>SHMQCIVNACKNSWDKSYLAGTPNKDNCSGFVQSVAAELGVPMPRGNANAMVDGLEQSWTKLASGAEAAQKAAQGFLVIAGLKGRTYGHVAVVISGPLYRQKYPMCWCGSIAGAVGQSQGLKSVGQVWNRTDRDRLNYYVYSLASC[2x];>[2x]ADCTFTQLEIVPQFGSPNMFGGEDEHVRVMFSNEDPNDDNPDAFPEPPVYLADRDSGNDCRIEDGGIWSRGGVFLSQDGRRVLMHEFSGSSAELVSYDSATCKVVHREDISGQRWAVDKDGLRLGQKC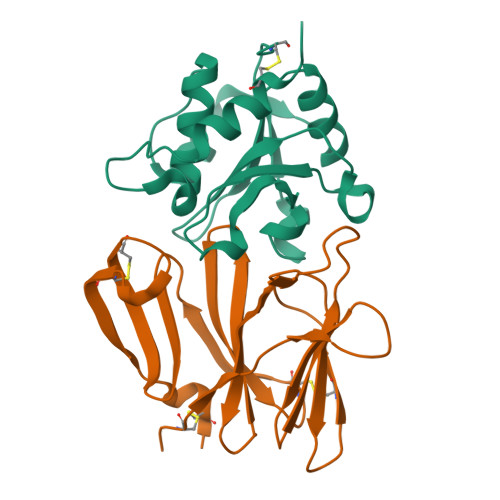SGESVDSCAKIVKRSLAPFCQTAKK> MRNKIFISHATPEDDDFTRWLSLKLIGLGYEVWCDILFLDKGVDFWSTIEKEIRENTCKFLIVSSTAGNKREGVLKELAVATKVKKHLQDDMFIIPLAIDENLSYDDINIEIVRLNAIDFKKSWAKGLQDLLDAFEKQNVPKKPPDHSKSNLLYQQIFLHDKQAIEKEETYDS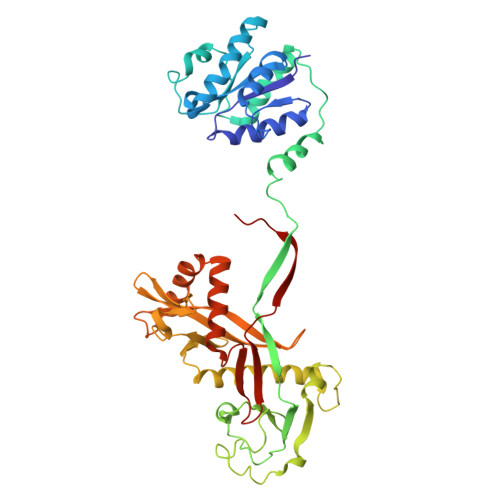NWFPIISFPNELRFHRYDWRLPKQFDVRTLAFPAIRYKEYLCTFAWEYDFIHQLPKTETYNGQESIRISTSDILSGRYDTDFIRNYECQRLIVQLINKAFELRMKDKNVREYQMSKTFAYWIEKGKLEKDKFEKIKLVGKQKNKYWHFGISAAGKLYPSPVLMVSSHIIFTMDGINLIKSKSIQHSSRRKQGKNWWNDKWREKLLAFIRFLSDDQNAIYLNVGSEEKILISNKPLKFFGKMSYVTPSE> GSHMASMKKKGSVAIVGRIILSGDTAYAQQTRGEEGAQEVSQTGRDKNEAEGEVQVLSTATQTFLGTCINGVMWTVFHGAGAKTLAGPKGPVVQMYTNVDKDLVGWPTPPGTRSLTP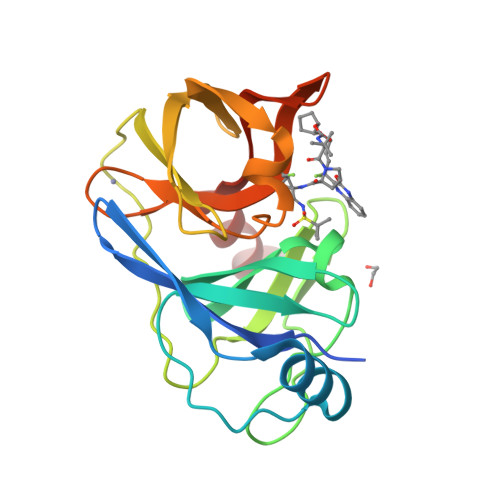CTCGSADLYLVTRHADVVPARRRGDTRASLLSPRPISYLKGSSGGPVMCPSGHVVGVFRAAVCTRGVAKALDFIPVENLETTMRSP> TTNNLQVTYPAPVAADGWEYRLISTGLTAPRSIVFDSTGGLLVLDAGVGVRRLTLQDNGGTCLSVTANATLIADTALNHGLAISADGGTIYASTVNDVYAYTYNEQTNTVDPTTRRTVVTNMTNTDHVTRTLLLSSRLPNELLVSRGSAANEDPQARNVTSGHSQIRAYDISTLAATDPPFDFVAGTLIGWGLRDSVGV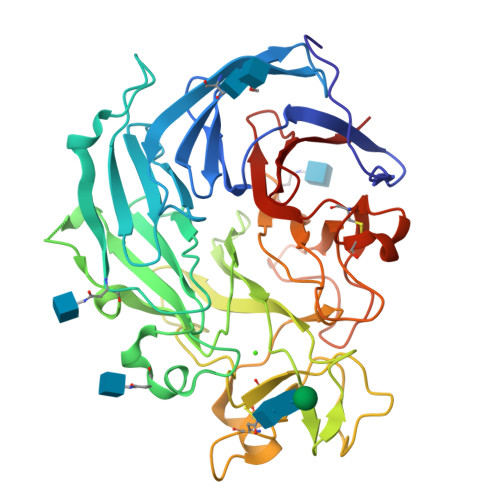GENPTNGGIWSVENSVDDLTREGVDVHQDNPGEELNFHGILGNTANQGGNYGYPDCYALWSTAGFPDLGALEVGDQFASDNATAGVTDATCNTNFVDPRLVFQAHVSPLDIKFNTNGTTAYITFHGSTDRTTPVGYSIVSVAFGLNGQPTSPMDSTTAANNILTSPDLTQCPDDCFTPVGLTFDTIGRLFFSSDSTGEIFVLQQS> MWPPRLLSCIFTIILIVAVIAPTSDSTTVRRRLRKPSKSVSVTSSVSRSTDQVISASVNRPKIRGRPSVASRKSSAALDNSVGTDDHKDKDGYKIVCYYTNWSQYRTKIGKFMPEDIQPELCTHIIFAFGWLKKGKLSSFESNDETKDGKTGLYDRINALKKANPKLKTLLAIGGWSFGTQKFKEMSATRYARQTFIYSAIPYLRDRNFDGLDIDWLYPKGGDDKKNYVLLLKELREAFEAEAQEVKKPRLLLTAAVPVGPDNIKSGYDVPAVASYLDFINLMAYDFHGKWERETGHNAPLYAPSSDSEWRKQLSVDHAAHLWVKLGAPKEKLIIGMPTYGRTFTLSNPNNFKVNSPASGGGKAGEYTKESGFLAYYEVCEILRNGGAYVWDDEMKVPYAIHGDQWVGFDDEKSIRNKMRWIKDNSFGGAMVWTVDMDDFSGGVCGGNVKYPLIGAMREELRGISRGKDAKDVDWASVAASV

Here, we report an arthropod-conserved insect chitinase belonging to group III from the pest Ostrinia furnacalis (OfChtIII), which contains two GH18 domains that act without synergism according to enzymatic assays and structural investigations. OfChtIII contains 987 amino-acid residues and is composed of four domains: a predicted TM domain (residues 7–29), two catalytic domains, GH18A (residues 94–461) and GH18B (residues 530–889), and a CBM14 domain (residues 922–976). The two GH18 domains of OfChtIII possess similar structures and substrate specificities, which differentiate them from the chitinolytic chitinase OfChtI-CAD. The degradation activity of GH18A and GH18B (or GH18B-CBM14) in combination towards EGC was equal to the activity calculated from the sum of the individual activities, suggesting that there was no synergistic effect between them.

In addition, the structures of two complexes were obtained: wild-type GH18A complexed with hydrolyzed (GlcNAc)6 and an active-site mutant, GH18A-E217L, complexed with intact (GlcNAc)6.>[2x]GGSGPLKPEEHEDILNKLLDPELAQSERTEALQQLRVNYGSFVSEYNDLTKEKSEFKLELDDVTSNMEQIIKAKANLEKMCRTLEDQMNEHRSKAEETQRSVN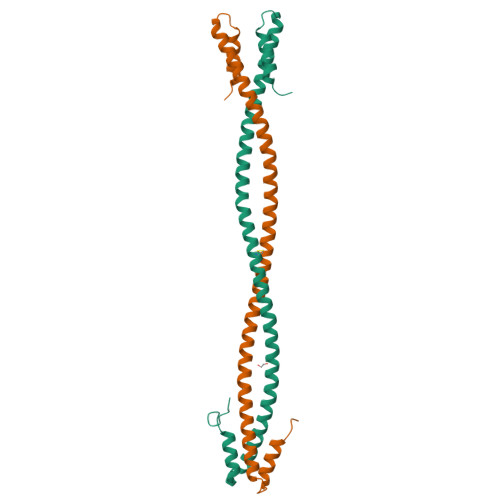DLTSQVEDLEKERDFYFGKLRNIELICQENEGENDPVLQRIVDILYATDEGFVIPD> MQEAARRASLRKEHTPTNEKFGDLSKQDSLGERASSKLTLDDELYDILYAFGETDAFINKGDKQRETDEDGNPLTRQALLERIRQKKEVIGKLRCQAWSMTRKRRTLKLAQKYLEQHESKVSRSHLYMEEMRKRARLMKRSFSNFKTYLIPWESKIKRIESHFGSVVSSYFTFLRWIVFVNIMITLIALVFVVLPETLADSVANEGRFNRTKTRKQIP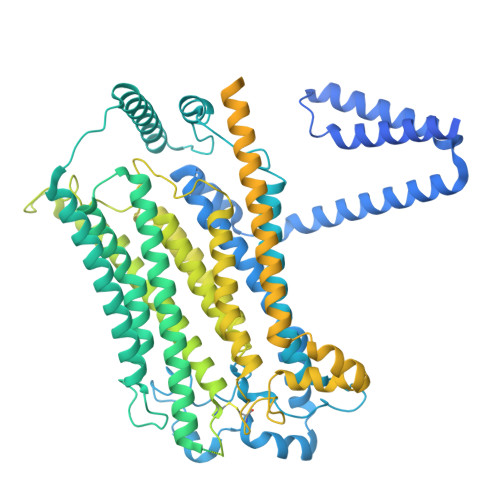ANERVHADELAVVWHYDGYLRYSPLFYGYYSDDPFLGNKIKYALPLAYFMVTLTIFAYSFFAILRKMAANARMSKLSGSKAEQYIFNWKLFTGWDYTIGNSETASNTVMAVVIKLRESIADIKKDAHGKFRLLQFSLRVFANIIICAMLGFSIYCIIFAVQKSQVQDDGNLFTKNQVPSVVSTITHVFPMIFDLIGKMENYHPRTALRAHLGRVLILYTVNYITLIFALFEKMTALRDRVNSTSTSSSHRTKRQQGGWNPNMQRPPPYASRAEVRQMSDFLAANTRRFQTVSQRTTRSVTTPFTVAPQFGPFNVNNPNAVFHNGTHSTSFESQILGPKALPIFTPPPRKYPGFTPGNVGQQFGGPDFPRNQVYTKSTPLPRVRTKPPWVYTTTHPPLVQNRAMTTTMSKSAKKGNSKNLDDDILLSNETIQMSEAALRRNHDGHNNDICWETIIGQEIVKLVTMDLIFTILSILVIDLFRGLWIKYCSSWWCWDIETTFPEYGEFKVAENVLHIINNQGMIWLGLFFAPLLPAINNIKLIILMYIRGWAVMTCNVPAREIFRASRSSNFYLGILLIWLLLCTLPVGFVIASMSPSRSCGPFARYQHFYTVVTREIEKRVDQTVLSYIRHIASPGVVIPIILFLILIIYFLFSLVRGLREANTDLQAQLVHERTEEKKKIFELAGGKKNKFEKDRDKKRSNDYIPLIEQRRREPWRQYHEMEADHALASDSSEESDINEDEDDERQPLTAYPLRAIETPPETLQVTAFHPSLGSLIENREMEDEESASGDQLPMIHKSVSFQGPSHMQMRQSISTESCSQISRSAIQVATPEEIRALLRPYLEAKYGIPYQHGIKSFPIDVHTPPNNTPSRRSSKYNSFVSLYEHTRDDHKNFVASTIKETDEDPGKSDKKQTSSKDVAPDFMPWPSADEARALREKMKSKTPLMLTKTTVEEKPKGGKSSESEFRPPVPIHRKYNIQTTEEENEEEETDSAPESSKKRFRISVSPTKTIAPASASRAQHKIVSQASSSSSIPHGRQPDPNKKASLVLPPLRAPRVQFDEDDSPRQID> SMSSFEGQMAEYPTISIDRFDRENLRARAYFLSHCDKDHMKGLRAPTLKRRLECSLKVYLYCSPVTKELLLTSPKYRFWKKRIISIEIETPTQISLVDEASGEKEEIVVTLLPAGHCPGSVMFLFQGNNGTVLYTGDFRLAQGEAARMELLHSGGRVKDIQSVYLDTTFCDPRFYQIPSREECLSGVLELVRSWITRSPYHVVWLNCKAAYGYEYLFTNLSEELGVQVHVNKLDMFRNMPEILHHLTTDRNTQIHACRHPKAEEYFQWSKLPCGITSRNRIPLHIISIKP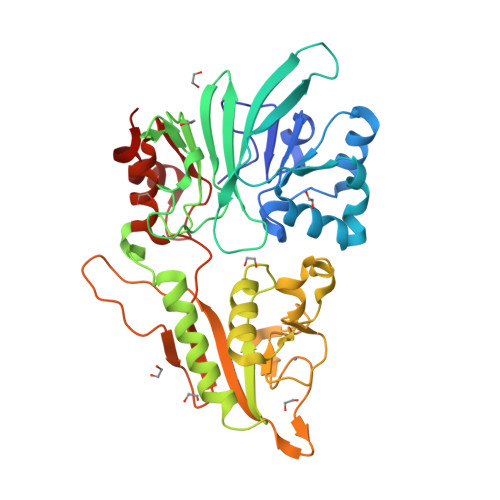STMWFGERSRKTNVIVRTGESSYRACFSFHSSYSEIKDFLSYLCPVNAYPNVIPVGTTMDKVVEILKPLCRS>MSFTPANRAYPYTRLRRNRRDDFSRRLVRENVLTVDDLILPVFVLDGVNQRESIPSMPGVERLSIDQLLIEAEEWVALGIPALALFPVTPVEKKSLDAAEAYNPEGIAQRATRALRERFPELGIITDVALDPFTTHGQDGILDDDGYVLNDVSIDVLVRQALSHAEAGAQVVAPSDMMDGRIGAIREALESAGHTNVRVMAYSAKYASAYYGPFRDAVGSASNLGKGNKATYQMDPANSDEALHEVAADLAEGADMVMVKPGMPYLDIVRRVKDEFRAPTFVYQVSGEYAMHMGAIQNGWLAESVILESLTAFKRAGADGI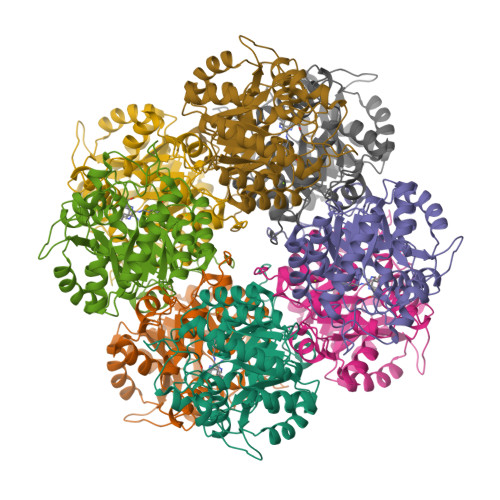LTYFAKQAAEQLRRGR[2x]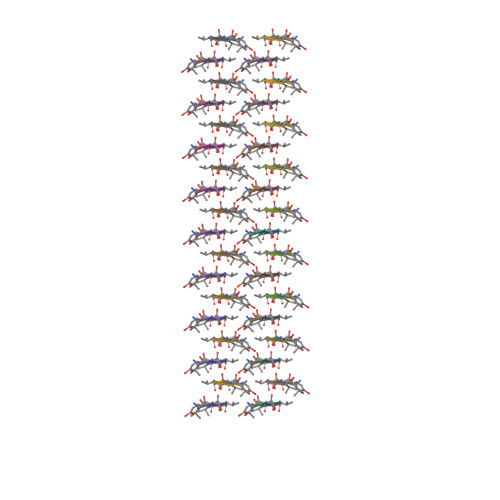> TSYVGV> GSTLQDDVRDGVAPNGSAQQLPQTIIIGVRKGGTRALLEMLSLHPDVAAAENEVHFFDWEEHYSHGLGWYLSQMPFSWPHQLTVEKTPAYFTSPKVPERVYSMNPSIRLLLILRDPSERVLSDYTQVFYNHMQKHKPYPSIEEFLVRDGRLNVDYKALNRSLYHVHMQNWLRFFPLRHIHIVDGDRLIRDPFPEIQKVERFLKLSPQINASNFYFNKTKGFYCLRDSGR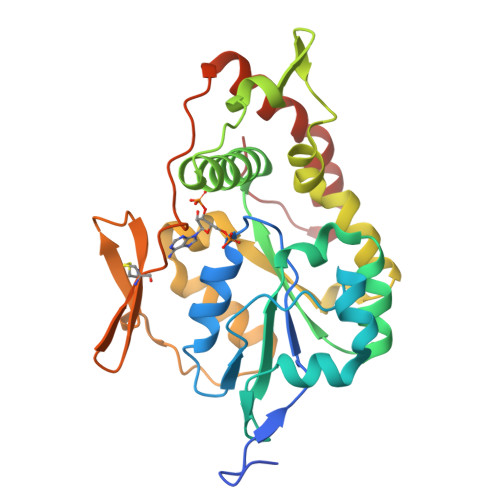DRCLHESKGRAHPQVDPKLLNKLHEYFHEPNKKFFELVGRTFDWH> AGVLLPVAYLGVRALEADPLVLREILLRPKNLELLRNTLGLAAGVLGLATLVALPAAYLTTRTDLRGKRLWATLLTLPLAVPGYVGAYVLLSATGPGGLLPLPRPEGYWGALLVLGLITYPYLFLALRAAFLGVDPSVEEAARTLGHPPWRVFLRVTLPQLLPAFLSGYLVIALHVLGDFGTVSLLRYETFSYAIYLQYSAAFDRVYAAWLALFLLLLTGSLLLLEAALLRRLSLGRTGRGAARTSPPARLGPLAPLAHLFLLLPFLLAVAFPLYALLHLARRFPASATSGLAEALGHALLVALPVAFLSVGMALPIAYLASRYPSAASRTLERLAYLAYAIPPLAYALAWIFFSLRT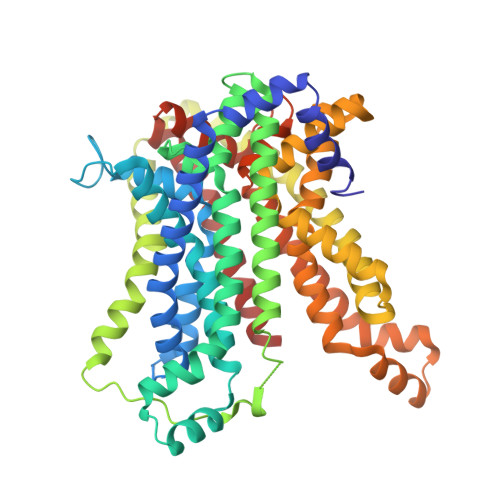LPFLYGTLALLVLALALHFLTESLGPVRSALAQVPPRLEEAARTLGDTPTRAFFRVTFPLLWRGAAAGGSLAFIGAMKELPITLLLAPTGFSTLATRVFGYTQEAMFAEAAPFALLIVGLSAAFVGVLLWNERRF In addition, the host intrinsic apoptosis pathway can be downregulated by viruses through the expression of B-cell lymphoma 2 (Bcl-2) mimics (vBcl-2), which nullify the activity of host cell apoptosis inducing Bcl-2 family members. Canarypox CNP058 is a vBcl-2 protein discovered amongst certain avipoxviruses. Our findings demonstrate that CNP058 is a Bcl-2 protein that potently inhibits apoptosis, is able to interact with the BH3 domain of pro-death Bcl-2 proteins, and provide a platform to understand apoptosis inhibition by CNP058. We showed that CNP058 binds to BH3 domains of pro-death proteins including Bak and Bax and most of the BH3-only proteins, and is able to protect HeLa cells against UV induced apoptosis. These findings establish CNP058 as a viral Bcl-2 protein with a broad pro-apoptotic Bcl-2 binding profile that is a potent inhibitor of apoptosis.

We then sought to understand the structural basis of CNP058 interaction with the BH3 domain of pro-death Bcl-2 by determining the structure of CNP058 in complex with the Bim BH3 domain. The CNP058-Bim BH3 domain complex structure revealed that CNP058 adopts the conserved Bcl-2-like fold consisting of eight α-helices and possessing the conserved hydrophobic groove found in other Bcl-2 family members that is utilized to accommodate Bim BH3 domain. The Bim BH3 domain is bound in the canonical hydrophobic ligand binding groove formed by α-helices 2–5. Detailed inspection of the CNP058-Bim BH3 domain complex interface showed that Bim residues Ile58, Leu62, Ile65 and Phe69 extend into four hydrophobic pockets on the CNP058 binding groove. In addition, two salt bridges are found at the interface: Asp83CNP058-Arg63Bim and the highly conserved Arg89CNP058-Asp67Bim, which is a hallmark of pro-survival Bcl-2:BH3 domain interactions. Notably, the highly conserved NWGR motif situated at the beginning of α5-helix of all Bcl-2 proteins is replaced with a TWGR motif in CNP058, however the Thr in the TWGR motif is not involved in any direct interactions with Bim. Furthermore, the substitution of an Asn in the highly conserved NWGR for Thr may cause the difference in the binding profile between the two avipoxvirus vBcl-2s, since the threonine in TWGR motif of CNP058 is unable to form hydrogen bonds with bound BH3 domains, whereas the corresponding Asn in FPV039 is involved in hydrogen bonds in complexes with Bik and Bmf. At the structural level, CNP058 possesses longer α4, α5, and α6 helices in comparison to FPV039. These topological differences may contribute to the distinct binding profiles of the two proteins as α4 and α5 helices form core segments of the hydrophobic binding groove. Interestingly, in CNP058, significant B-factor differences are observed for the entire α3 helix and the lower part of helix α4 compared to the central helix α5, suggesting that both α3 and α4 are display considerably higher flexibility.

> GPLGSMDPSVKKDEIYYTILNIIQNYFIEYCTGKNRNFHVEDENTYIIVKNMCDIILRDNIVEFRKDIDRCSDIENEIPEIVYDTIHDKITWGRVISIIAFGAYVTKVFKEKGRDNVVDLMPDIITESLLSRCRSWLSDQNCWDGLKA;> DMRPEIWIAQELRRIGDEFNAYYARR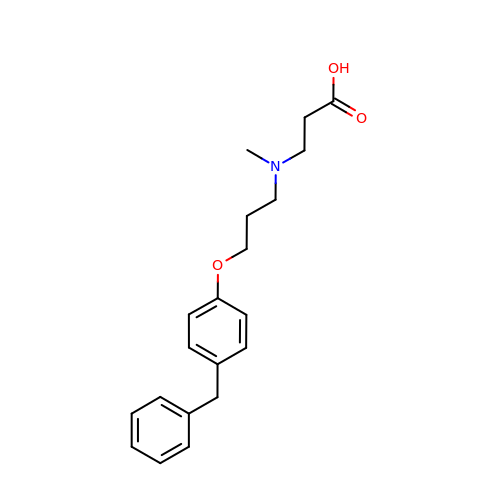N-[3-(4-benzylphenoxy)propyl]-N-methyl-beta-alanine | C20 H25 N O3 | HSXNVULMYZGNGF-UHFFFAOYSA-N>MANGTRQKDLRERAERVIPGGMYGHESTRLLPPEFPQFFRRALGARIWDADEQPYIDYMCAYGPNLLGYRQSEIEAAADAQRLLGDTMTGPSEIMVNLAEAFVGMVRHADWAMFCKNGSDATSTAMVLARAHTGRKTILCAKGAYHGASPWNTPHTAGILASDRVHVAYYTYNDAQSLSDAFKAHDGDIAAVFATPFRHEVFEDQALAQLEFARTARKCCDETGALLVVDDVRAGFRVARDCSWTHLGIEPDLSCWGKCFANGYPISALLGSNKARDAARDIFVTGSFWFSAVPMAAAIETLRIIRETPYLETLIASGAALRAGLEA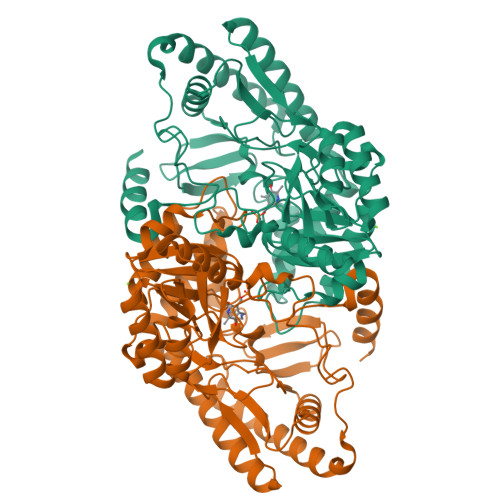QSQRHGLELKQTGPAQMPQIFFADDPDFRIGYAWAAACLKGGVYVHPYHNMFLSAAHTVDDVTETLEATDRAFSAVLRDFASLQPHPILMQLAGAASSVDKLAAALEHHHHHH[2x]(3S)-1-{[4-(BUT-2-YN-1-YLOXY)PHENYL]SULFONYL}PYRROLIDINE-3-THIOL | C14 H17 N O3 S2 | 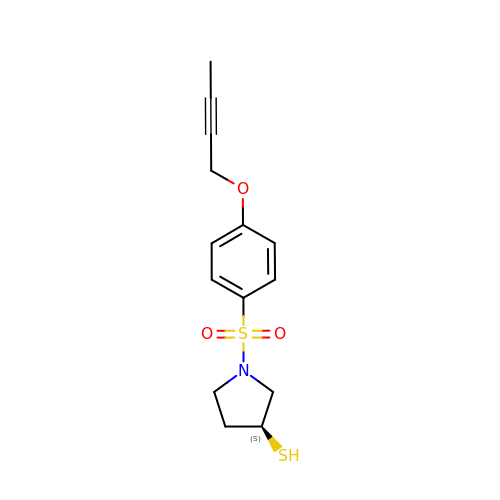BLIQFUCBRCDFAI-ZDUSSCGKSA-N> MATPSMLPQWAYMHIAGQDASEYLSPGLVQFARATDTYFSLGNKFRNPTVAPTHDVTTDRSQRLTLRFVPVDREDNTYSYKVRYTLAVGDNRVLDMASTYFDIRGVLDRGPSFKPYSGTAYNSLAPKGAPNSSQWEQKKAGNGDTMETHTFGVAPMGGENITIDGLQIGTDATADQDKPIYADKTFQPEPQVGEENWQETESFYGGRALKKDTSMKPCYGSYARPTNVKGGQAKLKVGADGVPTKEFDIDLAFFDTPGGTVNGQDEYKADIVMYTENTYLETPDTHVVYKPGKDDASSEINLVQQSMPNRPNYIGFRDNFIGLMYYNSTGNMGVLAGQASQLNAVVDLQDRNTELSYQLLLDSLGDRTRYFSMWNQAVDSYDPDVRIIENHGVEDELPNYCFPLDGSGTNAAYQGVKVKNGNDGDVESEWENDDTVAARNQLCKGNIFAMEINLQANLWRSFLYSNVALYLPDSYKYTPANITLPTNTNTYDYMNGRVVPPSLVDAYINIGARWSLDPMDNVNPFNHHRNAGLRYRSMLLGNGRYVPFHIQVPQK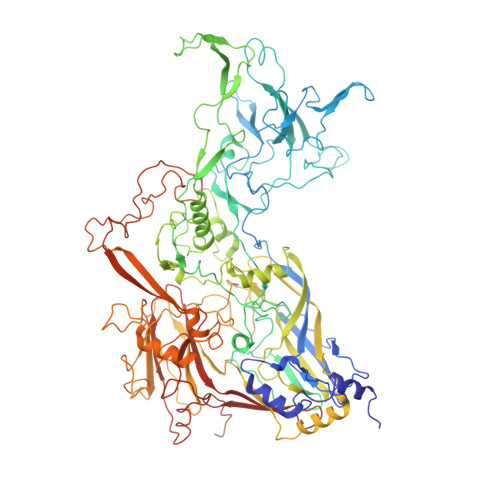FFAIKSLLLLPGSYTYEWNFRKDVNMILQSSLGNDLRTDGASISFTSINLYATFFPMAHNTASTLEAMLRNDTNDQSFNDYLSAANMLYPIPANATNVPISIPSRNWAAFRGWSFTRLKTKETPSLGSGFDPYFVYSGSIPYLDGTFYLNHTFKKVSITFDSSVSWPGNDRLLTPNEFEIKRTVDGEGYNVAQCNMTKDWFLVQMLAHYNIGYQGFYVPEGYKDRMYSFFRNFQPMSRQVVDEVNYKDYQAVTLAYQHNNSGFVGYLAPTMRQGQPYPANYPYPLIGKSAVTSVTQKKFLCDRVMWRIPFSSNFMSMGALTDLGQNMLYANSAHALDMNFEVDPMDESTLLYVVFEVFDVVRVHQPHRGVIEAVYLRTPFSAGNATT> TTIVSVRRNGHVVIAGDGQATLGNTVMKGNVKKVRRLYNDKVIAGFAG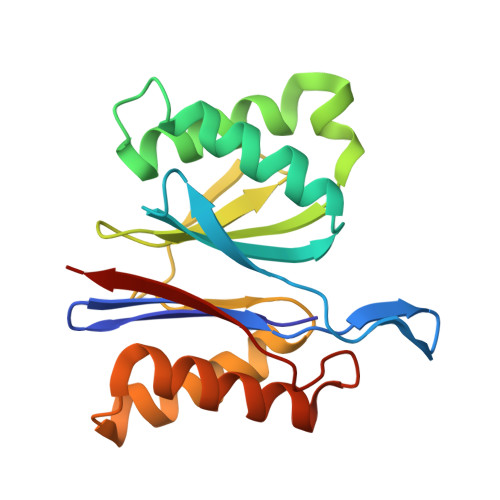GTADAFTLFELFERKLEMHQGHLVKAAVELAKDWRTDRMLRKLEALLAVADETASLIITGNGDVVQPENDLIAIGSGGPYAQAAARALLENTELSAREIAEKALDIAGDICIYTNHFHTIEELSYKA>MSDEQKKPEQIHRRDILKWGAMAGAAVAIGASGLGGLAPLVQTAAKPSKKDEKEEEQIVPFYGKHQAGITTAHQTYVYFAALDVTAKDKSDIITLFRNWTSLTQMLTSGKKMSAEQRNQYLPPQDTGESADLSPSNLTVTFGFGPGFFEKDGKDRFGLKSKKPKHLAALPAMPNDNLDEKQGGGDICIQVCADDEQVAFHALRNLLNQAVGTCEVRFVNKGFLSGGKNGETPRNLFGFKDGTGNQSTKDDTLMNSIVWIQSGEPDWMTGGTYMAFRKIKMFLEVWDRSSLKDQEDTFGRRKSSGAPFGQKKETDPVELNQIPSNPHVSLVKSTGKQILRRAFSYTE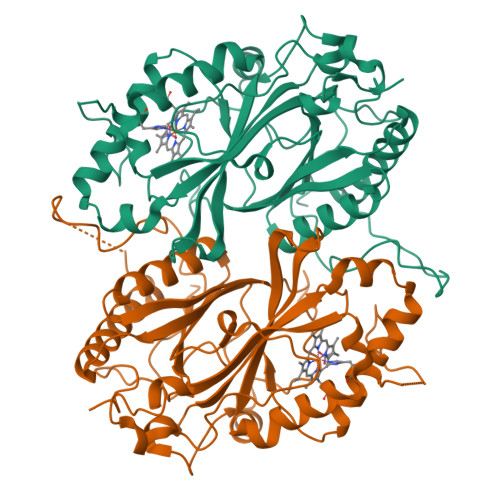GLDPKTGYMDAGLLFISFQKNPDNQFIPMLKALSAKDALNEYTQTIGSALYACPGGCKKGEYIAQRLLES[4x]>[4x]MEKAHPKEMVPLMGKRVAAPSGNPAILPEKRPAEITPTKKSAHFFLEIEGFEPNPTVAKTSPPVFSKPMDSNIRQCISGNCDDMDSPQSPQDDVTETPSNPNSPSAQLAKEEQRRKKRRLKKRIFAAVSEGCVEELVELLVELQELCRRRHDEDVPDFLMHKLTASDTGKTCLM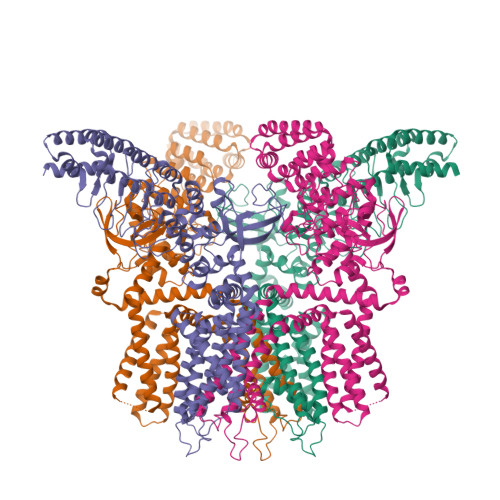KALLNINPNTKEIVRILLAFAEENDILGRFINAEYTEEAYEGQTALNIAIERRQGDIAALLIAAGADVNAHAKGAFFNPKYQHEGFYFGETPLALAACTNQPEIVQLLMEHEQTDITSRDSRGNNILHALVTVAEDFKTQNDFVKRMYDMILLRSGNWELETTRNNDGLTPLQLAAKMGKAEILKYILSREIKEKRLRSLSRKFTDWAYGPVSSSLYDLTNVDTTTDNSVLEITVYNTNIDNRHEMLTLEPLHTLLHMKWKKFAKHMFFLSFCFYFFYNITLTLVSYYRPREEEAIPHPLALTHKMGWLQLLGRMFVLIWAMCISVKEGIAIFLLRPSDLQSILSDAWFHFVFFIQAVLVILSVFLYLFAYKEYLACLVLAMALGWANMLYYTRGFQSMGMYSVMIQKVILHDVLKFLFVYIVFLLGFGVALASLIEKCPKDNKDCSSYGSFSDAVLELFKLTIGLGDLNIQQNSKYPILFLFLLITYVILTFVLLLNMLIALMGETVENVSKESERIWRLQRARTILEFEKMLPEWLRSRFRMGELCKVAEDDFRLCLRINEVKWTEWKTHVSFLNEDPGPVRRTDFNKIQDSSRNNSKTTLNAFEEVEEFPETSVVDAGLEVLFQGPAAAVDYKDDDDKAHHHHHHHHHH> SQCSSTLVKHIKAPLHLVWSIVRRFDEPQKYKPFISRCVVQGKKLEVGSVR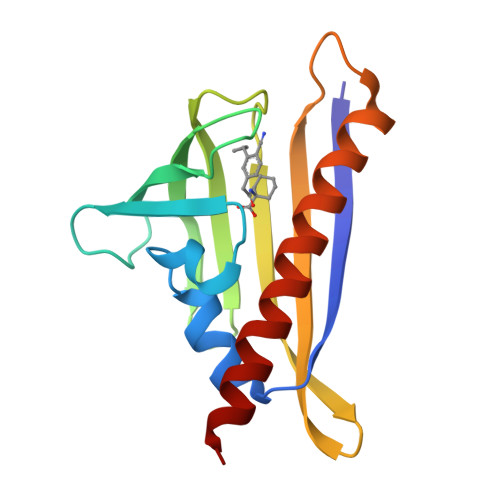EVDLKSGLPATKSTEVLEILDDNEHILGIRIVGGDHRLKNYSSTISLHSETIDGKTGTLAIESFVVDVPEGNTKEETCFFVEALIQCNLNSLADVTERLQAESM> GSKGRLVIYCSATNVMCENAAKTFEQKYDVKTSFIRNGSGSTFAKIEAEKNNPQADVWYGGTLDPQSQAGELGLLEAYRSPNIDQIMPKFQDPAKVKGNLSSAVYIGILGFAVNTERLKKLGIEKIPQCWNDLTDPKLKGEIQIADPQSSGTAYTAIATFAQLWGEDKAFDYFKHLHPNISQYTKSGITPARNAARGETTVGIGFLHDYALEKEQGAPLEMVVPCEG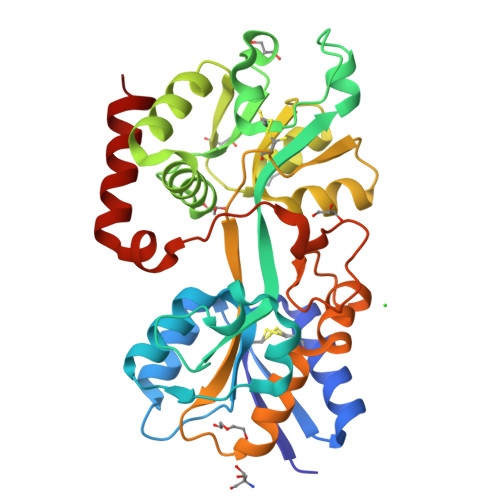TGYELGGVSILKGARNLDNAKLFVDFALSKEGQETAWKKGQALQTLTNTTAEQSPLAFDLTKLKLIDYDFEKYGASDERKRLINKWVDEIKLAK> ANIVGGIEYSINNASLCSVGFSVTRGATKGFVTAGHCGTVNATARIGGAVVGTFAARVFPGNDRAWVSLTSAQTL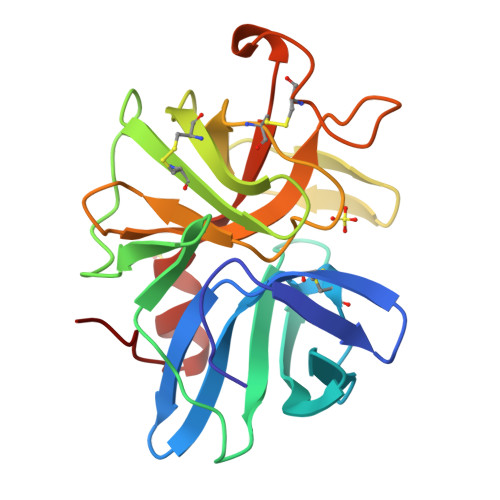LPRVANGSSFVTVRGSTEAAVGAAVCRSGRTTGYQCGTITAKNVTANYAEGAVRGLTQGNACAGRGDSGGSWITSAGQAQGVMSGANVQSNGNNCGIPASQRSSLFERLQPILSQYGLSLVTG> EKKFSTEEEYVSPRFLVADGFLIDLAEEKPINPKDPRLLTLLKDHQRAMIDQMNLVKWNDFKKYQD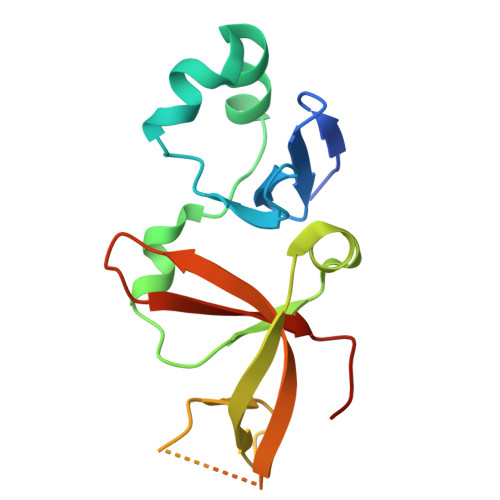PIPLKAKTLFKFCKQIKKKFLRGADFKLHTLPTEANLKYEPERMTVLCSCVPILLDDQTVQYLYDDSLEHHHHH>[2x]MLMVDEQLKIGATPMYSPSH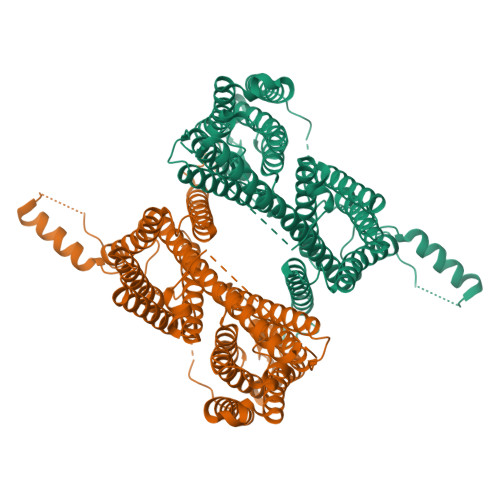NPIVIADDMEKGGSDSDSLPSSPTHHHELYRRPWIHEPRATNFFVRLITSLYALILTIISLVVEVSPTWRTDMWLAETIFYISMYGVGILFFAYCYIFIIYPGPYNQLISVLRKYKIIKNSEVWFIMQSQHNGEGAGTLYLRLGALFFGSVGIVLFGLELFLCIENVACKKVAIAKMIVAIVFTFIQMHFIFCNSKITVNSSRKIVAFGMMHLISVNLWTWFRFVLAKQEAKAHKKAQLKQTFRKYYSSSSSSSSEEIHELISAVLNSTLNNTPATKTMEPVASRLFALEHFGDVATFLTTCIVEYSLIGAAIMFILWKSIGQNNHQQSNSGKRKVKMRIDCSSSSTGLFAGIIFLIGSLVSMGMYTIFESLRNSSGAQLVFGIVDLSLFSIALGACIIGLWRMRHLQYRLHAHGEVIDEILLIIGLIGEILYCAVGIDVFITCRRSADLTVSALPAFVFVIRMIQVVVQAAFILTTSRLRCLSKYSMKYKPGKEIITFLLVSNVTLFVFHTFEGMKSSFGFSSKAATQYNYIIYAVGPLLVFYRFHSSACLAEIWKHTYSTKSNEYDHEHMSLSDSNLTAITPISDIKEIPSPQLLKH> KAFERCELARTLKRLGMDGYRGISLANWMCLAKWESGYNTRATNYNAGDRSTDYGIFQINSRYWCN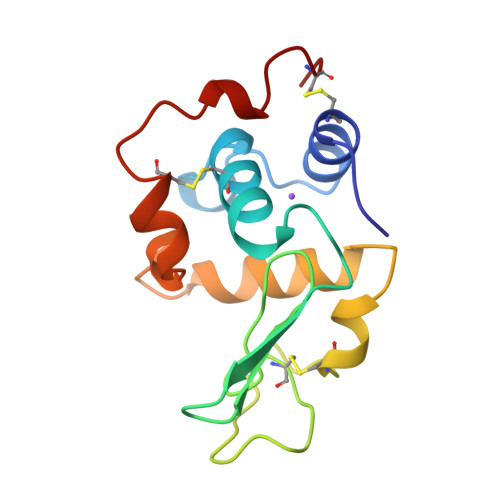DGKTPGAVNAAHLSCSALLQDNIADAVAAAKRVVRDPQGIRAWVAWRNRCQNRDVRQYVQGCGV> MAIATYNSHVELAKYLVSKADSVYLTIGKSTPWSNETNPPQPDENATVLQEVIGYK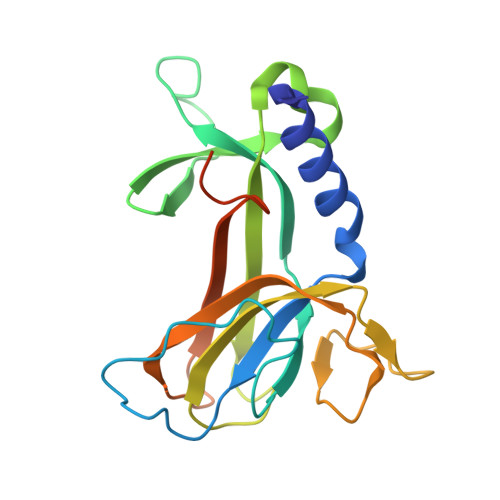KATKVTLVRPSKSPEDDNKNLISYGNKSWVEVTPENAKAEGAKWVYLESSIVGDELPLGTYRQVGFVMDLVAKSGISKFNLVPSEVESTGTLLFFDNKQFQNRSEQTTAKERFIVEVDPNSSSVDKLAAALEHHHHHH> APLVHHHHHHALDENLYFQGALADVSRPPHARKTGGSSPETKYDQPPKCDISGKEAISALSRAKSKHCRQEIGETYCRHKLGLLMPEKVTRFCPLEGKANKNVQWDEDSVEYMP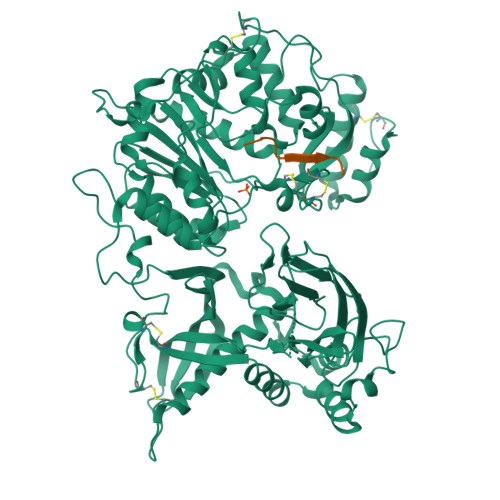ANPVRIAFVLVVHGRASRQLQRMFKAIYHKDHFYYIHVDKRSNYLHRQVLQVSRQYSNVRVTPWRMATIWGGASLLSTYLQSMRDLLEMTDWPWDFFINLSAADYPIRTNDQLVAFLSRYRDMNFLKSHGRDNARFIRKQGLDRLFLECDAHMWRLGDRRIPEGIAVDGGSDWFLLNRRFVEYVTFSTDDLVTKMKQFYSYTLLPAESFFHTVLENSPHCDTMVDNNLRITNWNRKLGCKCQYKHIVDWCGCSPNDFKPQDFHRFQQTARPTFFARKFEAVVNQEIIGQLDYYLYGNYPAGTPGLRSYWENVYDEPDGIHSLSDVTLTLYHSFARLGLRRAETSLHTDGENSCRYYPMGHPASVHLYFLADRFQGFLIKHHATNLAVSKLETLETWVMPKKVFKIASPPSDFGRLQFSEVGTDWDAKERLFRNFGGLLGPMDEPVGMQKWGKGPNVTVTVIWVDPVNVIAATYDILIESTAEFTHYKPPLNLPLRPGVWTVKILHHWVPVAETKFLVAPLTFSNRQPIKPEEALKLHNGPLRNAYMEQSFQSLNPVLSLPINPAQVEQARRNAASTGTALEGWLDSLVGGMWTAMDICATGPTACPVMQTCSQTAWSSFSPDPKSELGAVKPDGRLR;> QEEEGSAGGQGG> GDVEEAIDRAVARVADTMPTGPRNTESVPALTAVETGHTSQVVPGDTMQTRHVKNYHSRTESSIENFLCRAACVYIATYKSAGGTPTERYASWRINTRQMVQLRRKFELFTYLRFDMEITFVITSTQDPGTQLAQDMPVLTHQIMYIPPGGPVPNSATDFAWQSSTNPSIFWTEGCAPARMSVPFISIGNAYSNFYDGWSHFTQEGVYGFNSLNNMGHIYVRHVNEQSLGVSTSTLRVYFKPKHVRAWVPRPPRLSPYVKSSNVNFKPTAVTTERKDINDVGT;> SPTVEECGFSDRVRSITLGNSTITTQECANVVVGYGVWPSYLQDNEATAEDQPTQPDVATCRFYTLDSIQWQKESDGWWWKFPEALKNMGLFGQNMEYHYLGRSGYTIHVQCNASKFHQGCLLVVCVPEAEMGCSDVEREVVAASLSSEDTAKSFSRTESNGQHTVQTVVYNAGMGVGVGNLTIFPHQWINLRTNNSATIVMPYINSVPMDNMFRHYNFTLMIIPFAKLEYTEQASNYVPITVTVAPMCAEYNGLRLASHQ;> GLPTMLTPGSNQFLTSDDFQSPSAMPQFDVTPEMKIPGEVHNLMEIAEVDSVVPVNNTKENINSMEAYRIPVTGGDQLHTQVFGFQMQPGLNSVFKRTLLGEILNYYAHWSGSVKLTFVFCGSAMATGKFLLAYSPPGASPPQNRKQAMLGTHVIWDVGLQSSCVLCIPWISQTHYRLVQQDEYTSAGYVTCWYQTGLIVPPGAPPSCTILCFASACNDFSVRMLRDTPFIEQTQLLQ;> GAQVSTQKTGAHETSLTASGNSTIHYTNINYYKDAASNSANRQDFTQDPSKFTEPMKDVMIKSLPALN

The genus Enterovirus within the Picornaviridae, a family of non-enveloped viruses with a positive single-stranded RNA genome, is comprised of more than 100 serotypes. Human enteroviruses (EV) are presently classified into four groups, Enterovirus A-D (EV-A, B, C, and D), among which EV-B, the largest group, consists of over 60 serotypes, including all 6 serotypes of coxsackievirus B (CVB1-6), coxsackievirus A9 (CVA9), over 30 serotypes of echoviruses and more than 20 newly identified enteroviruses. The capsid proteins (VP1, VP2, and VP3) adopt the classical eight-stranded anti-parallel β-barrel configuration with the N-termini residing inside and the C-termini exposed on the surface. Most of the uncoating receptors bind to the “canyon” sites of the viral particle, dislodging the “pocket factor” in VP1 and subsequently triggering conformational changes of the intact particle to release the genome, albeit that SCARB2 binds EV71 outside the canyon.

Given that three key structural elements of the VP1 GH, VP2 EF, and VP1 EF loops dominate virus–receptor interactions, we systematically calculated pairwise Euclidean distances between all amino acids for all possible (n2) pairs of these three key elements from 15 structure-available human EVs, which defines a k (k = (n2)) dimensional space delineating the structural characteristics of the receptor-recognition sites. The phylogenetic tree could clearly separate these human EVs into three groups: EV-A, EV-B, and EV-C. Within each group, viruses with distinct receptors were further grouped into mono-phylogenetic clades. This structure-based in silico analysis completely matches the results of experimentally derived receptor identification, therefore, it can be used to deduce the receptor usage for human EVs. To test the robustness of our structure-based algorithm, we determined the structures of three other human EVs (CVB1, CVB5 and Echovirus 3) and put these into our algorithm. The in silico analysis suggests that CVB1 and CVB5 are CAR-dependent human EVs and E3 utilizes FcRn as a functional receptor, predictions consistent with experimental reports.> PASEQETLVRPKPLLLKLLKSVGAQK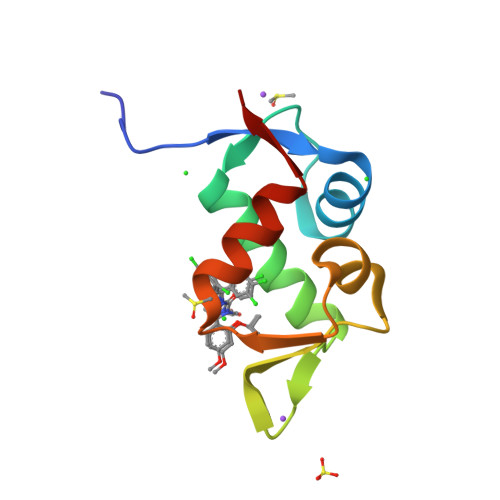DTYTMKEVLFYLGQYIMTKRLYDEKQQHIVYCSNDLLGDLFGVPSFSVKEHRKIYTMIYRNLVVVN> EERNDWHFNIGAMYEIENVEGYGEDMDGLAEPSVYFNAANGPWRIALAYYQEGPVDYSAGKRGTWF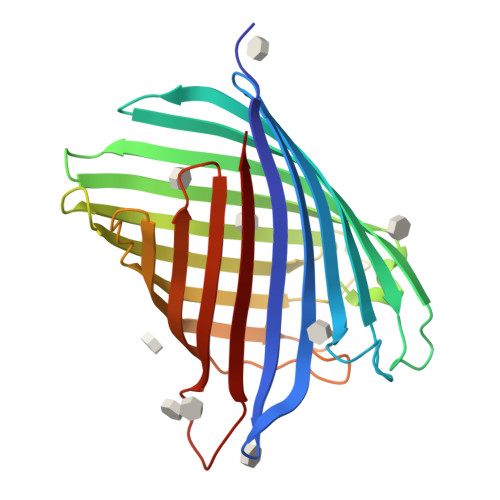DRPELEVHYQFLENDDFSFGLTGGFRNYGYHYVDEPGKDTANMQRWKIAPDWDVKLTDDLRFNGWLSMYKFANDLNTTGYADTRVETETGLQYTFNETVALRVNYYLERGFNMDDSRNNGEFSTQEIRAYLPLTLGNHSVTPYTRIGLDRWSNWDWQDDIEREGADFNRVGLFYGYDFQNGLSVSLEYAFEWQDADEGDSDKFHYAGVGVNYSF> GIGKFLHA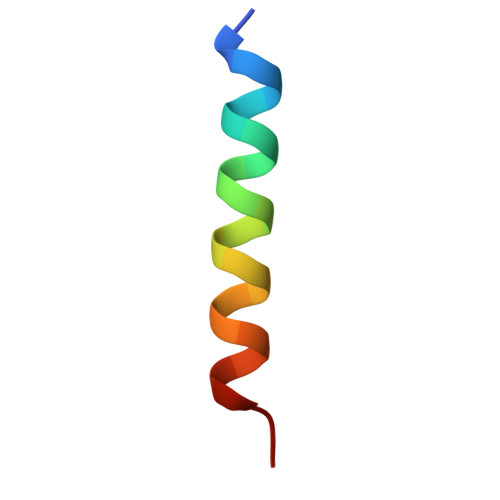AKKFAKAFVAEIMNS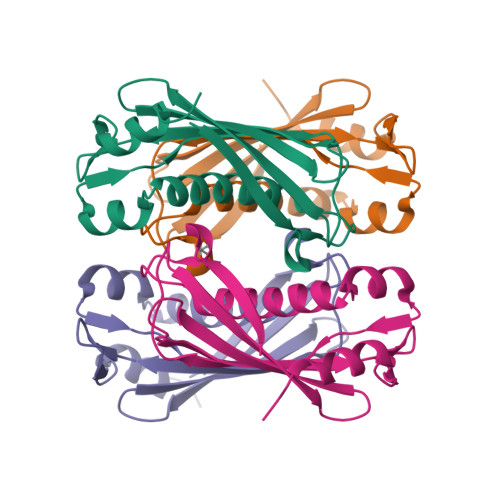>GSHMGTFTYERQVYLADTDGAGVVYFNQFLQMCHEAYESWLSSEHLSLQNIISVGDFALPLVHASIDFFAPAHCGDRLLVNLTITQASAHRFCCDYEISQAESAQLLARAQTHHVCIALPERKKAPLPQPWQTAICDLDHP[2x]>GMEVLDLVTGPDSVTEIEAFLNPRMGQPPTPESLTEGGQYYGWSRGINLATSDTEDSPENNTLPTWSMAKLQLPMLNEDLTCDTLQMWEAVSVKTEVVGSGSLLDVHGFNKPTDTVNTKGISTPV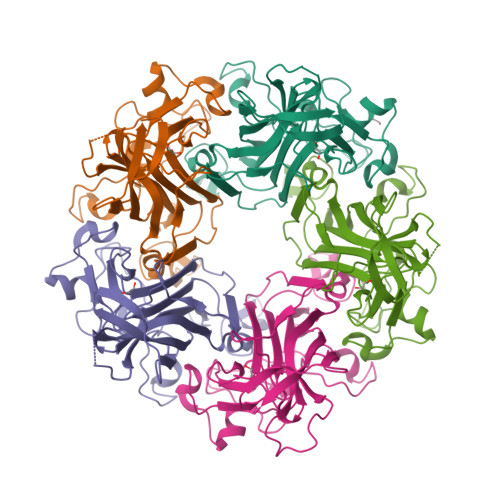EGSQYHVFAVGGEPLDLQGLVTDARTKYKEEGVVTIKTITKKDMVNKDQVLNPISKAKLDKDGMYPVEIWHPDPAKNENTRYFGNYTGGTTTPPVLQFTNTLTTVLLDENGVGPLCKGEGLYLSCVDIMGWRVTRNYDVHHWRGLPRYFKITLRKRWVK[5x]pyridin-2-amine | C5 H6 N2 | 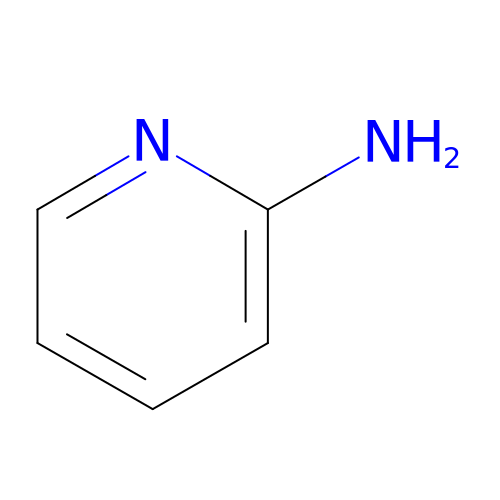ICSNLGPSRYBMBD-UHFFFAOYSA-N> MKMLLLLCLGLTLVCVHAEE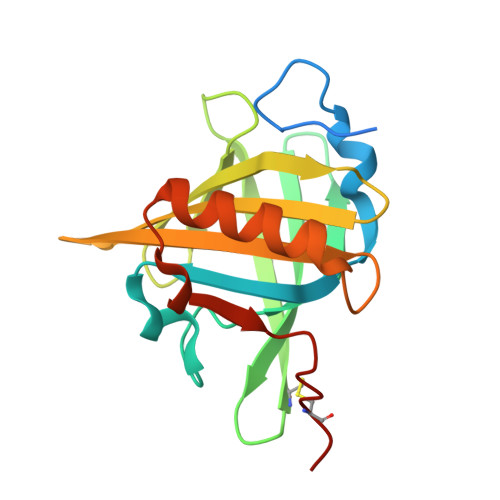ASSTGRNFNVEKINGEWHTIILASDKREKIEDNGNFRLFLEQIHVLENSLVLKFHTVRDEECSELSMVADKTEKAGEYSVTYDGFNTFTIPKTDYDNFLMAHLINEKDGETFQLMGLYGREPDLSSDIKERFAQLCEEHGILRENIIDLSNANRCLQARE The VEEV non-structural protein 2 (nsP2) is a cysteine protease (nsP2pro) that processes the polyprotein and thus it is a drug target for inhibitor discovery. The VEEV nsP2pro is a papain-like cysteine protease. The active enzyme consists of two subdomains; the N-terminal subdomain (which contains the active site residues C477 and H546) and the C-terminal SAM MTase subdomain that lacks enzymatic activity. The substrate binds in a cleft between the protease and the SAM MTase subdomains.

Here we report a high-resolution crystal structure of the VEEV nsP2pro, which contains the wild-type N475 residue at the N terminus and K741A/K767A surface entropy reduction mutations in the SAM Mtase domain distant from the active site. Surface entropy reduction mutations were introduced at residues K741 and K767 of the SAM MTase domain where the lysine residues were mutated to alanine. The goal of this modification was to obtain crystals that would diffract to high resolution for use in ligand soaking experiments and co-crystallization trials. The construct harboring the K741A/K767A mutations yielded crystals that diffracted to 1.46 A resolution. Inspection of the electron density maps revealed the presence of two conformations of the N-terminal oligopeptide residues prior to the catalytic C477. Electron density for the N-terminal residues was visible starting with K473 of the A’ (active, ~45% occupancy) conformer and N472 of the B’ (self-inhibited, ~55% occupancy) conformer. In the A’ (open) conformation, the N-terminal loop is exposed on the enzyme surface and the active site is accessible to substrate and ligands. In contrast, the B’ (closed) conformation reveals that the N-terminal residues 472AKANVC477 are flipped into the active site and to the interdomain cleft beneath the β-hairpin, thus acting as a pseudo-substrate. The B’ conformer of the K741A/K767A mutant nsP2pro construct used in our study was considered to be catalytically incompetent because the density for 472AKANVC477 is continuous and of high quality.

> RPDPTDVFQNKANVCWAKALVPVLKTAGIDMTTEQWNTVDYFETDKAHSAEIVLNQLCVRFFGLDLDSGLFSAPTVPLSIRNNHWDNSPSPNMYGLNKEVVRQLSRRYPQLPRAVATGRVYDMNTGTLRNYDPRINLVPVNRRLPHALVLHHNEHPQSDFSSFVSKLKGRTVLVVGEKLSVPGKMVDWLSDRPEATFRARLDLGIPGDVPKYDIIFVNVRTPYKYHHYQQCEDHAIKLSMLTKKACLHLNPGGTCVSIGYGYADRASESIIGAIARQFAFSRVCKPKSSLEETEVLFVFIGYDRAARTHNPYKLSSTLTNIYT JAK2, like other JAK family members, comprises a catalytically active C-terminal tyrosine kinase domain (JH1), a regulatory pseudokinase domain (JH2), and a Src homology-2 (SH2)-like domain that, together with the N-terminal FERM (N-terminal 4.1, ezrin, radixin, moesin) domain, forms the major receptor interaction moiety. The JH2 domain has a key role in mediating both negative and positive regulation of JAK kinase activity and numerous disease mutations locate in JH2, including the prevalent hyperactivating JAK2 V617F in MPN. Previous studies have demonstrated that JAK2 JH2 binds ATP and possesses regulatory autophosphorylation activity on Ser523 and Tyr570. To gain insights on the compound binding modes to JAK2 JH2 and to analyze whether any differences could be observed between binding to WT and V617F, we determined the crystal structures of selected small molecules with JAK2 JH2 WT and V617F.

Diaminotriazole compounds 16–21, in addition to primary hit 1, demonstrated substantial binding to JAK2 JH2 domain ATP-pocket, i.e., competition of fluorescent tracer was at or above 30% at 100 µM compound concentration. Compounds 16 and 19 engaged equally JH2 and JH1 domains, whereas analogs 17, 18, 20 and 21 possessed JH2-selective binding (2- to 3-fold). It should be noted that the conformation of the gatekeeper displays rather large variations in the structures, and it is unclear what the contribution of this interaction to the binding affinity is, especially since diaminotriazole analog 16, which also contains amide nitrogen at this position (actually even closer to the Gln626) does not make the gatekeeper H-bond. Since the compound binding does not induce significant changes in the ATP pocket, we compared the regions around residue 617 and the helix Cα between WT and V617F structures. It has been noted before that compound binding to JAK2 JH2 V617F can disrupt the aromatic packing of F617-F595-F594 and the conformation of F595 and F594 can be reverted back to the JAK2 JH2 WT conformation. In structures complexed with 6, 36, and 16, a WT-like conformation for the phenylalanines was observed. In the complexes with 36 and 16, the switch towards the WT-like conformation seems to start from the shifting of Gln626 gatekeeper position, which in turn affects the conformation of Leu624. This leucine forces both Phe594 and Phe595 to a new conformation. It appears to be possible to affect the conformation of the V617F region with small molecules, especially ones disturbing the position of the gatekeeper.

>VFHKIRNEDLIFNESLGQGTFTKIFKGVRREVGDYGQLHETEVLLKVLDKAHRNYSESFFEAASMMSKLSHKHLVLNYGVCFCGDENILVQEFVKFGSLDTYLKKNKNCINILWKLEVAKQLAAAMHFLEENTLIHGNVCAKNILLIREEDRKTGNPPFIKLSDPGISITVLPKDILQERIPWVPPECIENPKNLNLATDKWSFGTTLWEICSGGDKPLSALDSQRKLQFYEDRHQLPAPKAAELANLINNCMDYEPDHRPSFRAIIRDLNSLFTPDLVPRGSHHHHHH[2x]>GHHHHHHELANNTTGFTRIIKAAGYSWKGLRAAWINEAAFRQEGVAVLLAVVIACWLDVDACTRVLLISSVMLVMIVELLNSAIEAVVDRIGSEYHELSGRAKDLGSAAVLIAIIDAVITWCILLWSHFG[3x]

Diacylglycerol kinase (DgkA) is the smallest known kinase. In Escherichia coli, it is responsible for the adenosine triphosphate (ATP)-dependent phosphorylation of diacylglycerol (DAG) to phosphatidic acid used in periplasm membrane-derived oligosaccharide synthesis in response to osmotic shock1. The enzyme has long served as a model for integral membrane enzymology, folding456, assembly and stability. It is a trimer with three active sites of the shared sites type that exhibits moderate positive heteroallostery, random-binding kinetics and lipid substrate promiscuity. Each subunit has four helices, three of which are largely membrane embedded (H1-3), whereas the fourth, an N-terminal amphiphilic surface helix (SH), anchors the protein at the membrane interface.

Therefore, the enzyme was co-crystallized with the non-hydrolysable ATP analogue, adenylylmethylenediphosphonate (ACP). Best crystals, providing a ternary complex structure with ACP and lipid bound at 2.7 Å resolution, were obtained with Δ4-DgkA grown in 9.9 MAG at 4 °C and soaked with zinc-ACP. Like the apo-enzyme, the ternary complex is a homo-trimer. In the complex, asBC has zinc-ACP and lipid bound. The zinc-ACP is close to fully extended and is secured by electrostatic, hydrogen bonding and hydrophobic interactions along its length on the relatively flat, cytosol-exposed surface of H2C and H3C. The two zinc atoms (Zn1, Zn2) bound to ACP were identified and positioned in the complex by anomalous scattering. They are bidentately coordinated, respectively, by the β- and γ- and the α- and γ-phosphates of ACP and fasten the polyphosphate to conserved residues Glu28C and Glu76C in the active site in ways that make catalytic sense. The two hydroxyls of ribose in ACP are tightly hydrogen bonded to the side-chain carboxyl of the essential Asp95C. The purine ring of ACP is locked in position by hydrogen bonds between the N1 and N6 of adenine and the backbone linkage of His87C and Glu85C, respectively, in CLC. MAG1 has been modelled into the electron density map with its headgroup deep in the protein positioned at the level of the membrane interface with its reactive 1-OH next to the γ-phosphate of ACP. Further, the γ-phosphate of ATP should be proximal to the 1-OH of the lipid substrate. This is what was observed in the ternary complex where the two entities are poised for reaction ∼4 Å apart.> 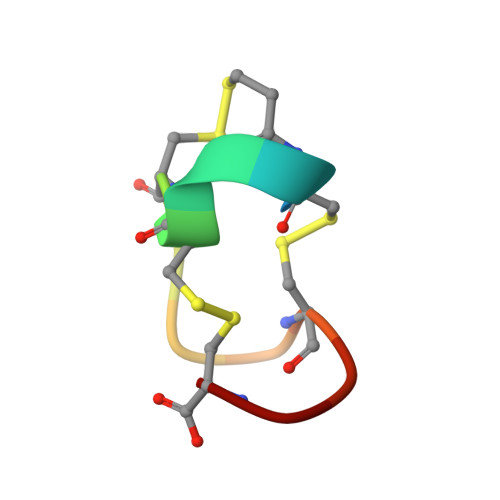XCELCCNPACAGC> LKESPSGYLRSGEGDTGCGELVWVGEPLTLRTAETITGKYGVWMRDPKPTYPYTQETTWRIDTVGTDVRQVFEYDLISQFMQGYPSKVHILPRPLESTGAVVYSGSLYFQGAESRTVIRYELNTETVKAEKEIPGAGYHGQFPYSWGGYTDIDLAVDEAGLWVIYSTDEAKGAIVLSKLNPENLELEQTWET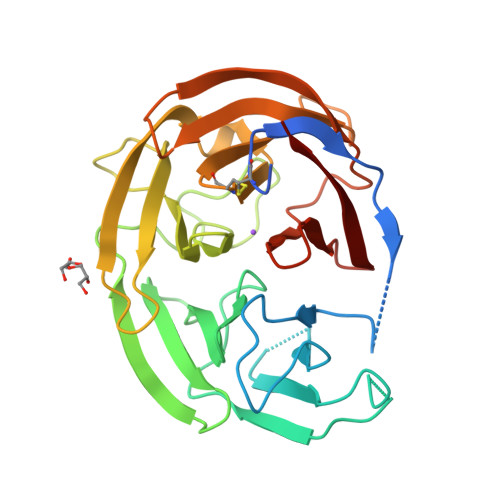NIRKQSVANAFIICGTLYTVSSYTSADATVNFAYDTGTGISKTLTIPFKNRYKYSSMISYNPLEKKLFAWDNLNMVTYDIKLSKM(3,3-dimethylpiperidin-1-yl)(6-(3-fluoro-4-methylphenyl)pyridin-2-yl)methanone 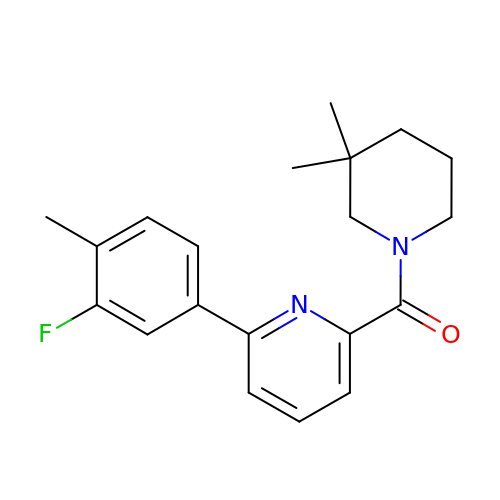| C20 H23 F N2 O | SIDDLTBLAQYZIZ-UHFFFAOYSA-N>GPADTLQSLAILGATGSIGDSTLAIIRQHPNRYRIHALTGFSRVDKLLALAMEFHPVKICTSPDNYAQLSQKVTDAGLDTIILSGDEGLIEIASDEAVDTVVAAIVGAAGLSSTLAAAGAGKRILLANKESLVMAGDLVIKTAKKHGATILPIDSEHNAIYQCLPAAIQADNTAIHHTSYGIKKLWLTASGGSFLDKSIKQMQNASVKEAVNHPNWSMGQKISIDSATMMNKGLELIEACHLFDLKEHQIQVVIHPNSVVHSLVEYVDGSFLAQLGTPDMKTPIAHALAYPERIKSGVMPLD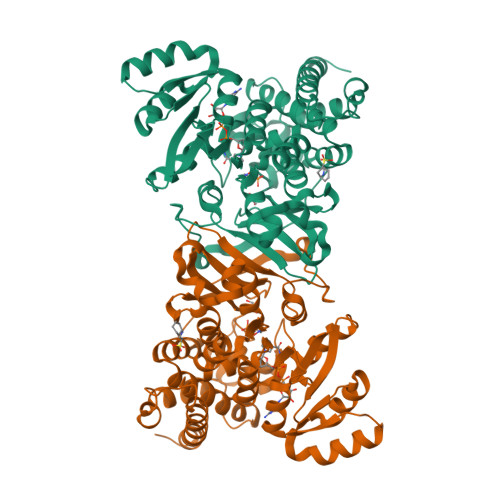LYQLGSLKFLAPDLDKFACLKLARYAARLGTGACIALNTANEIAVEAFLAEKICLTDIAVIVKACLDDKTIAQDYSQDFGDEVLGLERILTMDKKVRKIATAKIKLLKQGDVL[2x]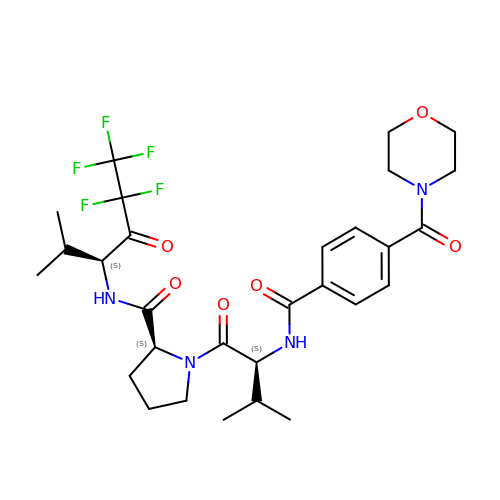1-{3-METHYL-2-[4-(MORPHOLINE-4-CARBONYL)-BENZOYLAMINO]-BUTYRYL}-PYRROLIDINE-2-CARBOXYLIC ACID (3,3,4,4,4-PENTAFLUORO-1-ISOPROPYL-2-OXO-BUTYL)-AMIDE | C29 H37 F5 N4 O6 | XQAMVCHQGHAELT-FKBYEOEOSA-N>[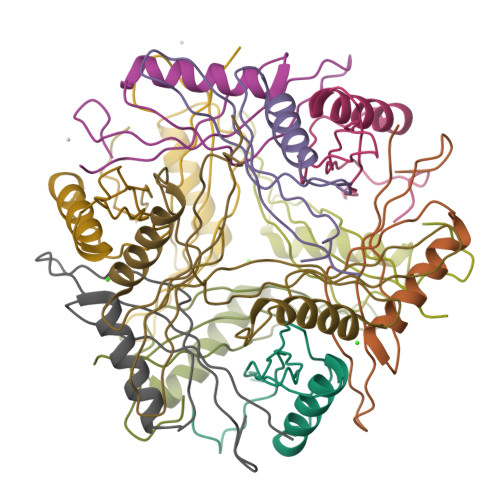12x]MVSVYKVIDIIGTSPTSWEQAAAEAVQRARDSVDDIRVARVIEQDMAVDSAGKITYRIKLEVSFKMRPSQPL>MAVESRSRVTSKLVKAHRAMLNSVTQEDLKVDRLPGADYPNPSKKYSSRTEFRDKTDYIMYNPRPRDEPSSENPVSVSPLLCELAAARSRIHFNPTETTIGIVTCGGICPGLNDVIRSITLTGINVYNVKRVIGFRFGYWGLSKKGSQTAIELHRGRVTNIHHYGGTILGSSRGPQDPKEMVDTLERLGVNILFTVGGDGTQRGALVISQEAKRRGVDISVFGVPKTIDNDLSFSHRTFGFQTAVEKAVQAIRAAYAE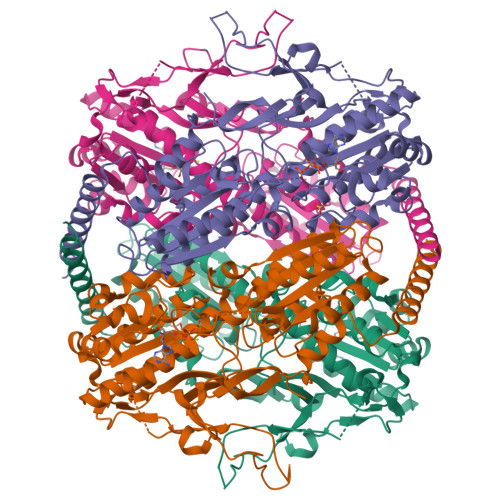AVSANYGVGVVKLMGRDSGFIAAQAAVASAQANICLVPENPISEQEVMSLLERRFCHSRSCVIIVAEGFGQDWGRGSGGYDASGNKKLIDIGVILTEKVKAFLKANKSRYPDSTVKYIDPSYMIRACPPSANDALFCATLATLAVHEAMAGATGCIIAMRHNNYILVPIKVATSVRRVLDLRGQLWRQVREITVDLGSDVRLARKLEIRRELEAINRNRDRLHEELAKL[4x]>[2x]AGQQQPLPVPPLLESRRGQPLFMTVQRAHW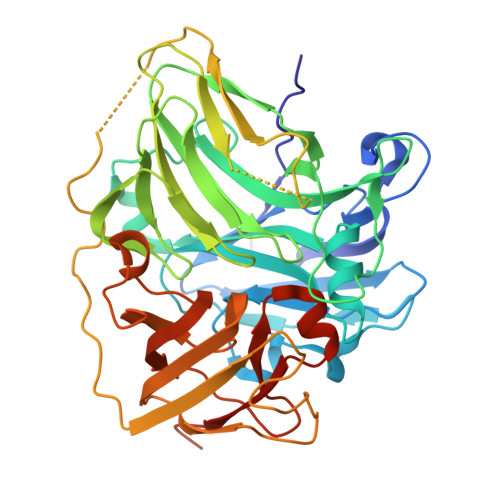SFTPGTRASVWGINGRYLGPTIRVWKGDDVKLIYSNRLTENVSMTVAGLQVPGPLMGGPARMMSPNADWAPVLPIRQNAATLWYHANTPNRTAQQVYNGLAGMWLVEDEVSKSLPIPNHYGVDDFPVIIQDKRLDNFGTPEYNEPGSGGFVGDTLLVNGVQSPYVEVSRGWVRLRLLNASNSRRYQLQMNDGRPLHVISGDQGFLPAPVSVKQLSLAPGERREILVDMSNGDEVSITCGEAASIVDRIRGFFEPSSILVSTLVLTLRPTGLLPLVTDSLPMRLLPTEIMAGSPIRSRDISLGDDPGINGQLWDVNRIDVTAQQGTWERWTVRADEPQAFHIEGVMFQIRNVNGAMPFPEDRGWKDTVWVDGQVELLVYFGQPSWAHFPFYFNSQTLEMADRGSIGQLLVNPVPRSHHHHHH> DALKVNRAPVGVEPQEVHKWLQSFNWDFKENRTKYPTKYHMANETKEQFKVIAKEYARMEAAKDERQFGTLLDGLTRLGAGNKVHPRWGETMKVISNFLEVGEYNAIAASAMLWDSATAAEQKNGYLAQVLDEIRHTHQCAFINHYYSKHYHDPAGHNDARRTRAIGPLWKGMKRVFADGFISGDAVECSVNLQLVGEACFTNPLIVAVTEWASANGDEITPTVFLSVETDELRHMANGYQTVVSIANDPASAKFLNTDLNNAFWTQQKYFTPVLGYLFEYGSKFKVEPWVKTWNRWVYEDWGGIWIGRLGKYGVESPASLRDAKRDAYWAHHDLALAAYAMWPLGFARLALPDEEDQAWFEANYPGWADHYGKIFNEWKKLGYEDPKSGFIPYQWLLANGHDVYIDRVSQVPFIPSLAKGTGSLRVHEFNGKKHSLTDDWGERQWLIEPERYECHNVFEQYEGRELSEVIAEGHGVR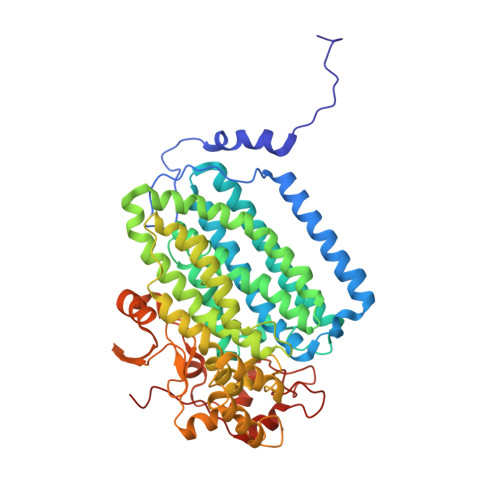SDGKTLIAQPHTRGDNLWTLEDIKRAGCVFPDPLAKF>ARSYGNGVYCNNKKCWVNRGEATQSIIGGMISGWASGLAGM[3x];>MKHHHHHHHGAAGTSLYKKAGENLYFQGSMKADYKKINSILTYTSTALKNPKIIKDKDLVVLLTIIQEEAKQNRIFYDYKRKFRPAVTRFTIDNNFEIPDCLVKLLSAVETPKAWSGFS[3x];>MDLNFIQVILVIFVAFLAGVEGILDQFHFHQPVIACTLIGLVTGNLLPCLILGGTLQMIALGWANVGAAVAPDAALASIASAIILVLGGQGKAGVTSAIAIAVPLAVAGLLLTIIVRTLATGIVHIMDAAAKEGNFRKIEMWQYIAIIMQGVRIAIPAGLILAIGAGPVKEMLTAMPVWLTDGLAIGGGMVVAVGYAMVINMMATKEVWPFFAIGFVLATISQLTLIGLGAIGISLALIYLALSKQGSGNNGGGSNTGDPLGDIIDNY[3x];>MAEQLKLTKKDRISVWLRSTFLQGSWNYERMQNGGWAYTLIPALKKLYKTKEDRSAALVRHMEFFNTHPYVAAPILGVTLALEEERANGAPIDDVTIQGVKVGMMGPLAGIGDPVFWFTVKPIIGALAASLAMSGNILGPIIYFVAWNAIRMAFTWYTQEFGYRAGSKITED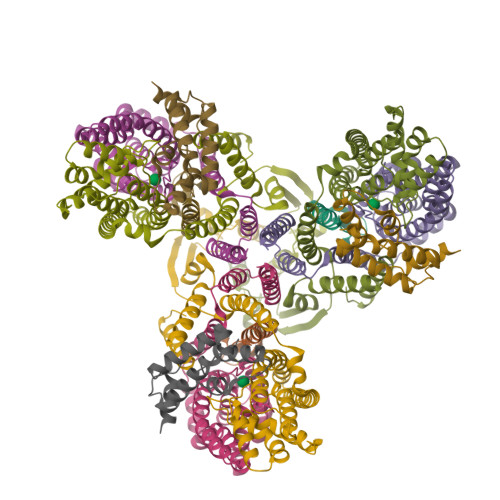LSGGILQDITKGASILGMFILGSLVNRWVSVKFTPTVSSVKLDKGAFIDWDKLPSGAKGIQSALQQQAQGLSLTDHKITTLQDNLDSLIPGLAALGLTLFCMWLLKKKVSPIVIILGLFVVGIVFHLLHLM[3x]> MAQNLKDLAGRLPAGPRGMGTALKLLLGAGAVAYGVRESVFTVEGGHRAIFFNRIGGVQQDTILAEGLHFRIPWFQYPIIYDIRARPRKISSPTGSKDLQMVN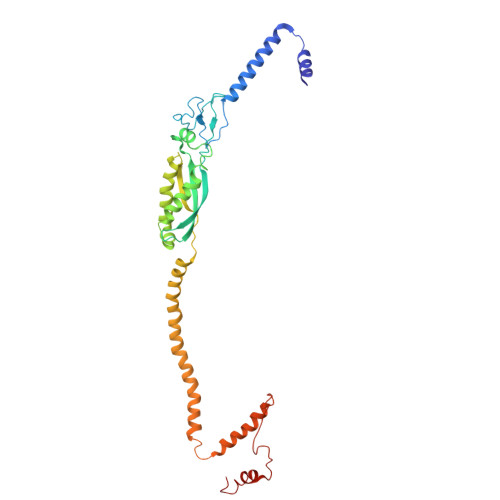ISLRVLSRPNAQELPSMYQRLGLDYEERVLPSIVNEVLKSVVAKFNASQLITQRAQVSLLIRRELTERAKDFSLILDDVAITELSFSREYTAAVEAKQVAQQEAQRAQFLVEKAKQEQRQKIVQAEGEAEAAKMLGEALSKNPGYIKLRKIRAAQNISKTIATSQNRIYLTADNLVLNLQDESFTRGSDSLIKGKK> MASAAGVRSTRQ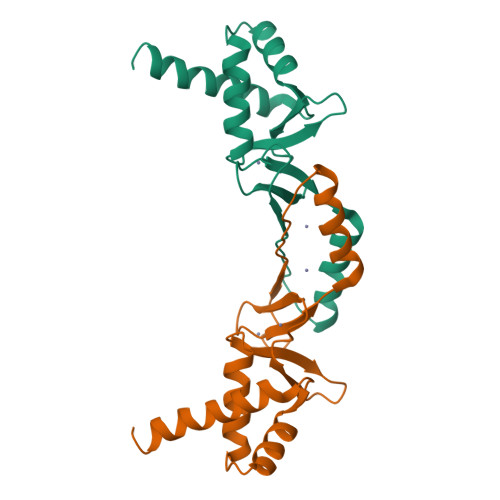RAAISTLLETLDDFRSAQELHDELRRRGENIGLTTVYRTLQSMASSGLVDTLHTDTGESVYRRCSEHHHHHLVCRSCGSTIEVGDHEVEAWAAEVATKHGFSDVSHTIEIFGTCSDCRS> U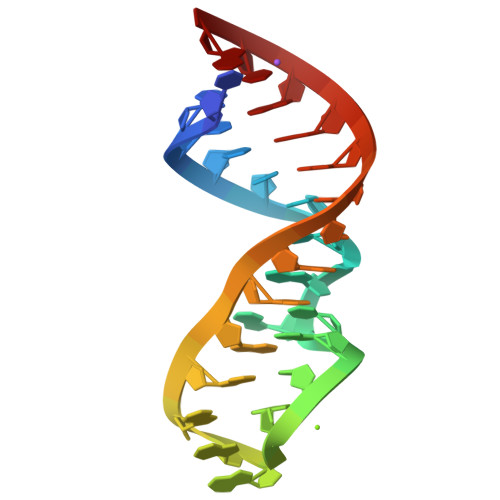GCUCCUAGUACGAGAGGAACGGAGUG> DYPKALQ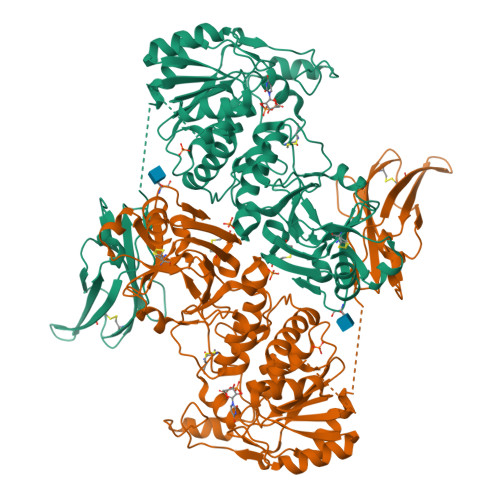ILMEGGTHMVCTGRTHTDRICRFKWLCYSNEAEEFIFFHGNTSVMLPNLGSRRFQPALLDLSTVEDHNTQYFNFVELPAAALRFMPKPVFVPDVALIANRFNPDNLMHVFHDDLLPLFYTLRQFPGLAHEARLFFMEGWGEGAHFDLYKLLSPKQPLLRAQLKTLGRLLCFSHAFVGLSKITTWYQYGFVQPQGPKANILVSGNEIRQFARFMTEKLNVSHTGVPLGEEYILVFSRTQNRLILNEAELLLALAQEFQMKTVTVSLEDHTFADVVRLVSNASMLVSMHGAQLVTTLFLPRGATVVELFPYAVNPDHYTPYKTLAMLPGMDLQYVAWRNMMPENTVTHPERPWDQGGITHLDRAEQARILQSREVPRHLCCRNPEWLFRIYQDTKVDIPSLIQTIRRVVKGRPGPRKQKWTVGLYPGKVREARCQASVHGASEARLTVSWQIPWNLKYLKVREVKYEVWLQEQGENTYVPYILALQNHTFTENIKPFTTYLVWVRCIFNKILLGPFADVLVCNT> GPMEDVEIKPRGYQLRLVDHLTKSNGIVYLPTGSGKTFVAILVLKRFSQDFDKPIESGGKRALFMCNTVELARQQAMAVRRCTNFKVGFYVGEQGVDDWTRGMWSDEIKKNQVLVGTAQVFLDMVTQTYVALSSLSVVIIDECHHGTGHHPFREFMRLFTIANQTKLPRVVGLTGVLIKGNEITNVATKLKELEITYRGNIITVSDTKEMENVMLYATKPTEVMVSFPHQEQVLTVTRLISAEIEKFYVSLDLMNIGVQPIRRSKSLQCLRDPSKKSFVKQLFNDFLYQMKEYGIYAASIAIISLIVEFDIKRRQAETLSVKLMHRTALTLCEKIRHLLVQKLQDMTYDDDDDNVNTEEVIMNFSTPKVQRFLMSLKVSFADKDPKDICCLVFVERRYTCKCIYGLLLNYIQSTPELRNVLTPQFMVGRNNISPDFESVLERKWQKSAIQQFRDGNANLMICSSVLEEGIDVQACNHVFILDPVKTFNMYVQSKGRARTTEAKFVLFTADKEREKTIQQIYQYRKAHNDIAEYLKDRVLEKTEPELYEIKGHFQDDIDPFTNENGAVLLPNNALAILHRYCQTIPTDAFGFVIPWFHVLQEDERDRIFGVSAKGKHVISINMPVNCMLRDTIYSDPMDNVKTAKISAAFKACKVLYSLGELNERFVPKTLKERVASIADVHFEHWNKYGDSVTATVNKADKSKDRTYKTECPLEFYDALPRVGEICYAYEIFLEPQFESCEYTEHMYLNLQTPRNYAILLRNKLPRLAEMPLFSNQGKLHVRVANAPLEVIIQNSEQLELLHQFHGMVFRDILKIWHPFFVLDRRSKENSYLVVPLILGAGEQKCFDWELMTNFRRLPQSHGSNVQQREQQPAPRPEDFEGKIVTQWYANYDKPMLVTKVHRELTPLSYMEKNQQDKTYYEFTMSKYGNRIGDVVHKDKFMIEVRDLTEQLTFYVHNRGKFNAKSKAKMKVILIPELCFNFNFPGDLWLKLIFLPSILNRMYFLLHAEALRKRFNTYLNLHLLPFNGTDYMPRPLEIDYSLKRNVDPLGNVIPTEDIEEPKSLLEPMPTKSIEASVANLEITEFENPWQKYMEPVDLSRNLLSTYPVELDYYYHFSVGNVCEMNEMDFEDKEYWAKNQFHMPTGNIYGNRTPAKTNANVPALMPSKPTVRGKVKPLLILQKTVSKEHITPAEQGEFLAAITASSAADVFDMERLEILGASFLKLSATLYLASKYSDWNEGTLTEVKSKLVSNRNLLFCLIDADIPKTLNTIQFTPRYTWLPPGISLPHNVLALWRENPEFAKIIGPHNLRDLALGDEESLVKGNCSDINYNRFVEGCRANGQSFYAGADFSSEVNFCVGLVTIPNKVIADTLEALLGVIVKNYGLQHAFKMLEYFKICRADIDKPLTQLLNLELGGKKMRANVNTTEIDGFLINHYYLEKNLGYTFKDRRYLLQALTHPSYPTNRITGSYQELEFIGAAILDFLISAYIFENNTKMNPGALTDLRSALVNNTTLACICVRHRLHFFILAENAKLSEIISKFVNFQESQGHRVTNYVRILLEEADVQPTPLDLDDELDMTELPHANKCISQEAEKGVPPKGEFNMSTNVDVPKALGDVLEALIAAVYLDCRDLQRTWEVIFNLFEPELQEFTRKVPINHIRQLVEHKHAKPVFSSPIVEGETVMVSCQFTCMEKTIKV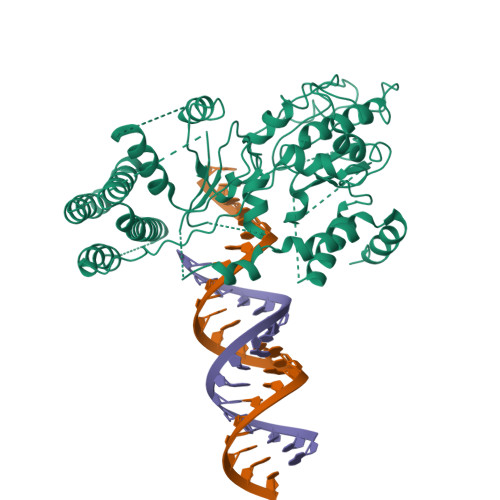YGFGSNKDQAKLSAAKHALQQLSKCDA>SNASPPQKVCLICGDEASGCHYGVLTCGSCK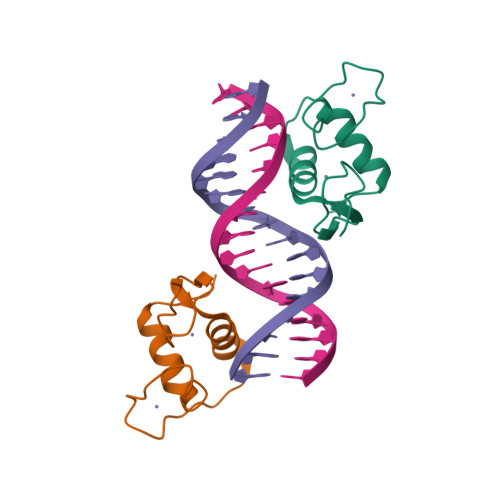VFFKRAVEGQHNYLCAGRNDCIIDKIRRKNCPACRLRKCLQAGMTLGARKSKKL[2x]>GSHMASKPIEDYGKGKGRIEPMYIPDNTFYNADDFLVPPHCKPYIDKILLPGGLVKDRVEKLAYDIHRTYFGEELHIICILKGSRGFFNLLIDYLATIQKYSGRESSVPPFFEHYVRLKSYQNDNSTGQLTVLSDDLSIFRDKHVLIVEDIVDTGFTLTEFGERLKAVGPKSMRIATLVEKRTDRSNSLKGDFVGFSIEDVWIVGCCYDFNEMFRDFDHVAVLSDAARKKF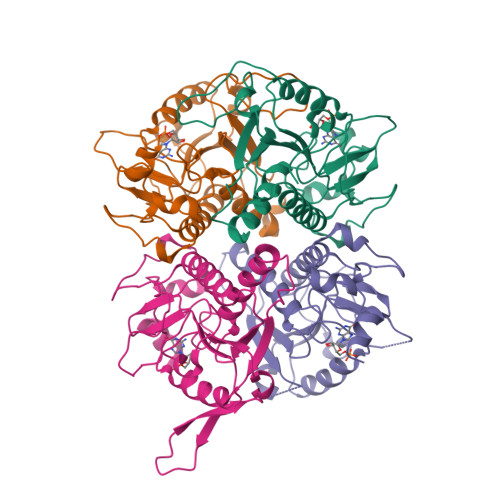EK[4x]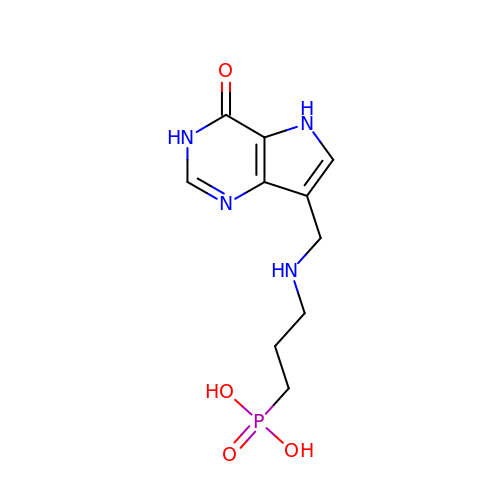(3-{[(4-oxo-4,5-dihydro-3H-pyrrolo[3,2-d]pyrimidin-7-yl)methyl]amino}propyl)phosphonic acid | C10 H15 N4 O4 P | BYPYXSLOGVUHEY-UHFFFAOYSA-N> MRRYEVNIVLNPNLDQ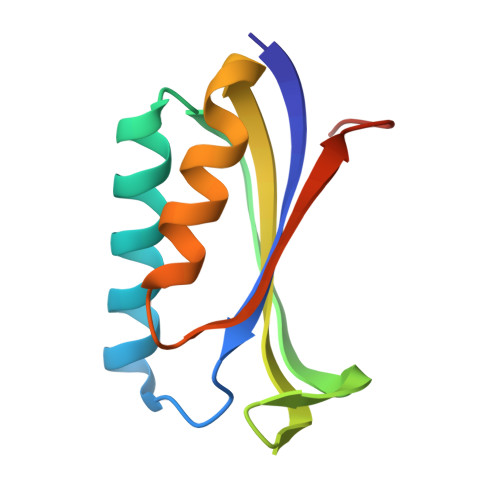SQLALEKEIIQRAAENYGARVEKVEELGLRRLAYPIAKDPQGYFLWYQVEMPEDRVNDLARELRIRDNVRRVMVVKSQEPFLANA>GEYKMMMARVAALPEDYQFVFKKIQNYMWNFSAGNGMDMLHIQYELIDLFEAGAAEGRQVLDITGEDV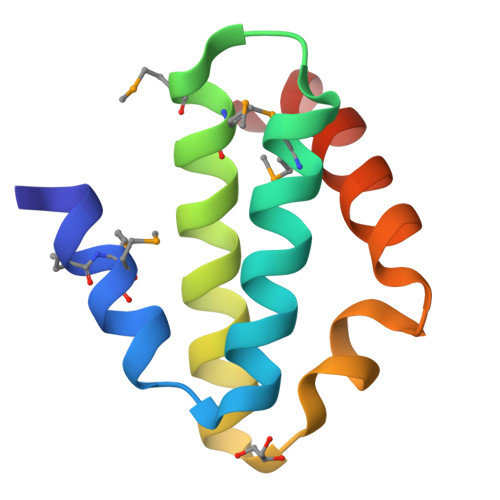ASFADELVANAKTYVSK[2x]>[6x]MNKNRGFTPLAVVLMLSGSLALTGCDDKQAQQGGQQMPAVGVVTVKTEPLQITTELPGRTSAYRIAEVRPQVSGIILKRNFKEGSDIEAGVSLYQIDPATYQATYDSAKGDLAKAQAAANIAQLTVNRYQKLLGTQYISKQEYDQALADAQQANAAVTAAKAAVETARINLAYTKVTSPISGRIGKSNVTEGALVQNGQATALATVQQLDPIYVDVTQSSNDFLRLKQELANGTLKQENGKAKVSLITSDGIKFPQDGTLEFSDVTVDQTTGSITLRAIFPNPDHTLLPGMFVRARLEEGLNPNAILVPQQGVTRTPRGDATVLVVGADDKVETRPIVASQAIGDKWLVTEGLKAGDRVVISGLQKVRPGVQVKAQEVTADNNQQAASGAQPEQSKS;>MKKLLPILIGLSLSGFSSLSQAENLMQVYQQARLSNPELRKSAADRDAAFEKINEARSPLLPQLGLGADYTYSNGYRDANGINSNATSASLQLTQSIFDMSKWRALTLQEKAAGIQDVTYQTDQQTLILNTATAYFNVLNAIDVLSYTQAQKEAIYRQLDQTTQRFNVGLVAITDVQNARAQYDTVLANEVTARNNLDNAVEQLRQITGNYYPELAALNVENFKTDKPQPVNALLKEAEKRNLSLLQARLSQDLAREQIRQAQDGHLPTLDLTASTGISDTSYSGSKTRGAAGTQYDDSNMGQNKVGLSFSLPIYQGGMVNSQVKQAQYNFVGASEQLESAHRSVVQTVRSSFNNINASISSINAYKQAVVSAQSSLDAMEAGYSVGTRTIVDVLDATTTLYNAKQELANARYNYLINQLNIKSALGTLNEQDLLALNNALSKPVSTNPENVAPQTPEQNAIADGYAPDSPAPVVQQTSARTTTSNGHNPFRN[3x];>MRYSKLTMLIPCALLLSACTTVTPAYKDNGTRSGPCVEGGPDNVAQQFYDYRILHRSNDITALRPY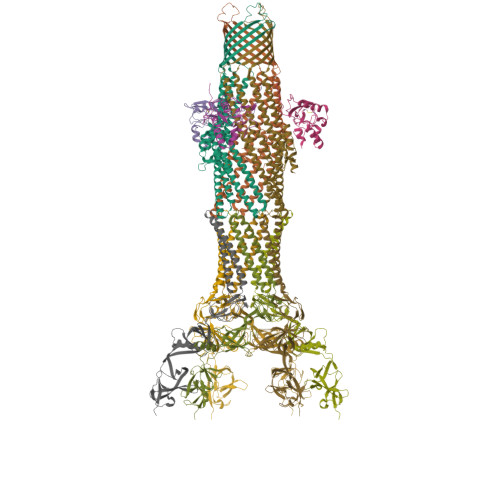LSDKLATLLSDASRDNNHRELLTNDPFSSRTTLPDSAHVASASTIPNRDARNIPLRVDLKQGDQGWQDEVLMIQEGQCWVIDDVRYLGGSVHATAGTLRQSIENR[3x]>[2x]MKDFKEIEIILDIIKTTREIIEDNDNDNEKISYHRNNIRKSIFFLQEELLEKYSET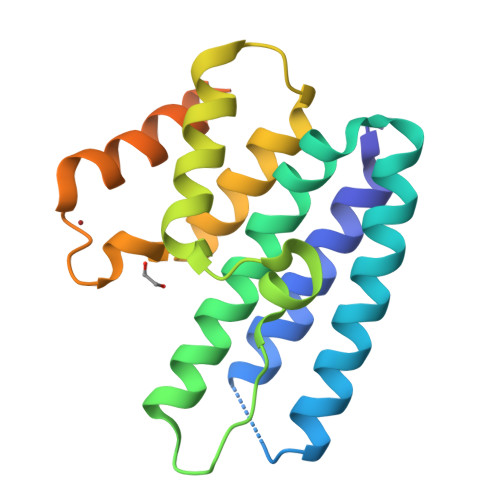VCKYIVFPLLAYVDEKLMLLREKSASNISWSLLQLEYYDRKDGGEYVFEITDNILSENIYPQICYQTISLILHNDFYGKYYDNIYNHSFLAYKKEIDKHIENSTIDSVNFIDIPVNSPPLSRKYSKTLK>MGGLLFSSLQHCQQGFVISNELRQQQSELTSTWDLMLQTRINLSRSAARMMMDASNQQSSAKTDLLQNAKTTLAQAAAHYANFKNMTPLPAMAEASANVDEKYQRYQAALAELIQFLDNGNMDAYFAQPTQGMQNALGEALGNYARVSENLYRQTFDQS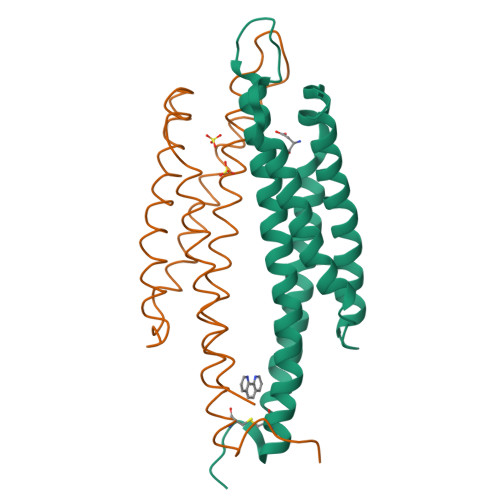AHDYR[2x]> GMTMKTRDKILLSSLELFNDKGERNITTNHIAAHLAISPGNLYYHFRNKSDIIYEIFQEYEKLVDYYLDIPEDRPITLEDMTFYLESVFDGLWSYRFFHRDLEYLLDSDPRLRQDYREFTNRCLAAINRIFAKLADAGIIQPQPEDLRSAMSLNVWLVITNWMAFLKTAHAAEEPASLSLTELKQGIYQVLTLEVPYLTPEYRERVLALREKY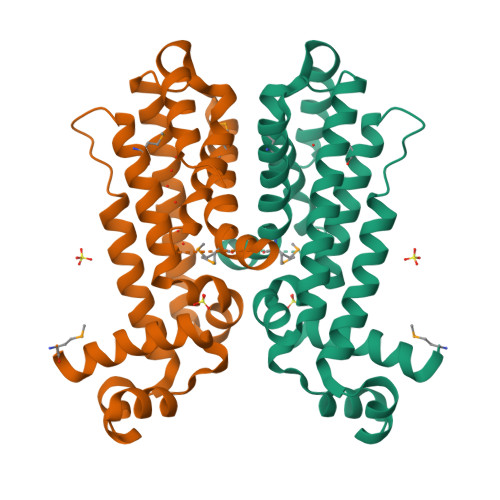RPTLPEAQGISGVEA>MAATTVNGGTVHFKGEVVNAACAVDAGSVDQTVQLGQVRT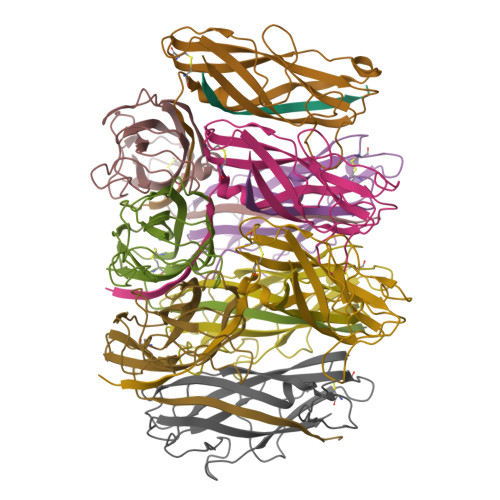ASLAQEGATSSAVGFNIQLNDCDTNVASKAAVAFLGTAIDAGHTNVLALQSSAAGSATNVGVQILDRTGAALTLDGATFSSETTLNNGTNTIPFQARYFATGAATPGAANADATFKVQYQ[10x]> KLKEKENNDSSDKATVIPNFNTTMQGSLLGDDSRDYYSFEVKEEGEVNIELDKKDEFGVTWTLHPESNIND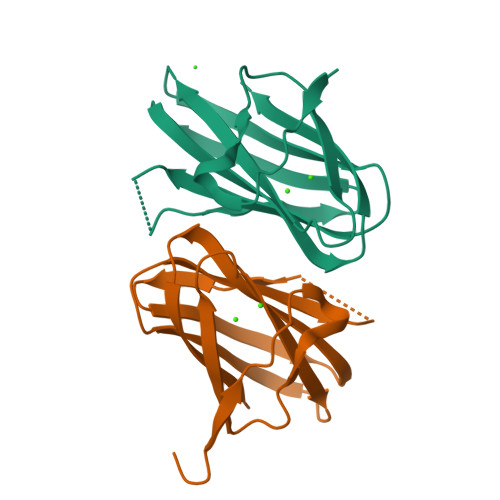RITYGQVDGNKVSNKVKLRPGKYYLLVYKYSGSGNYELRVNK;> IPGNEKLKEKENNDSSDKATVIPNFNTTMQGSLLGDDSRDYYSFEVKEEGEVNIELDKKDEFGVTWTLHPESNINDRITYGQVDGNKVSNKVKLRPGKYYLLVYKYSGSGNYELRVNK> SHMANKREPAPGWPIVSGEYVVGNPESCVGVVTLGSHGLEQACIDAGAAIAGPCHTENLGIEKVVANYISNPNIRFMILCGSEVQGHITGQCFKALWENGIGDDGGIIGAKG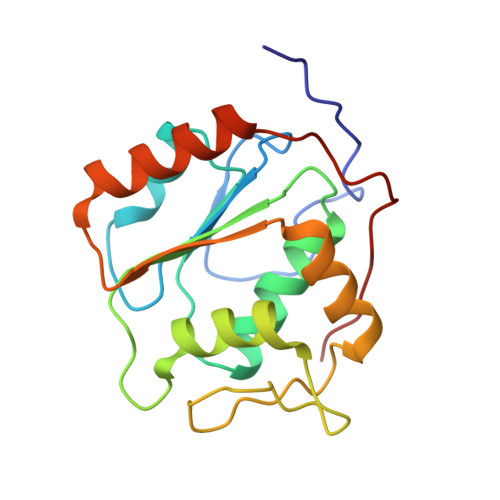AIPFLENVNKEAVERFRRQIVEVVDLIDCEDIGKITQAIKECLSKDPGAIDEDPFIIELE> SNKVGTLQAQVEATQKQKAQPI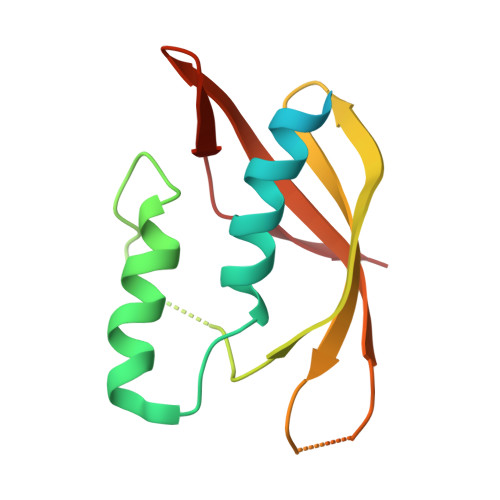DANRKYDYKLQYYLNDYVYAYFTLPQEGDKQQAQVEHLNSFYNFVPDVKAQGQVRNPSTLLDSQLVTVEGKVATYKVKYKEMIQHDKDTEEKELVTGFNIPFDEKEGKYYVSGLPWFSA>[4x]MAHHHHHHMLNDPEARMVANCPVLVTGGARRIGKAIVEDLASHGFPVAIHCNRSLDEGEAIANRINDSGGNACVVQADLEGDVRGLVKQASDRIGPIRLLVNNASLFQEDKVGALDMALWDRHFAVHLKTPVILAEDMRKALPED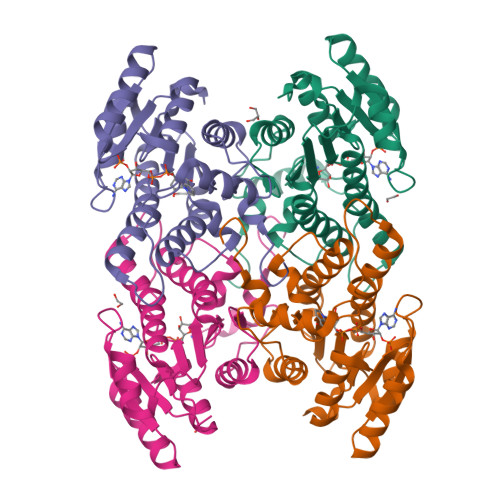QDGLVVNIIDQRVWKLNPQFFSYTLSKSALWNATRTLAQALAPRIRVNAIAPGPTLPSERQRPEDFERQVSKLPLQRAPELPEFGRTVRYFWENRSITGQMIALDGGQHLAWETPDIAGITE> SMFLQRPKPYSDESLESFFIRVANKNGYGDVHRFLEATKRFLQDIDHNGYQTFPTDITRINPYSAKNSSSARTASFLKLAQLTFNEPPELLGLAINRTNMKYSPSTSAVVRGAEVFPRSLLRTHSIPCCPLCLRENGYASYLWHFQGYEYCHSHNVPLITTCSCGKEFDYRVSGLKGICCKCKEPITLTSRENGHEAACTVSNWLAGHESKPLPNLPKSYRWGLVHWWMGIKDSEFDHFSFVQFFSNWPRSFH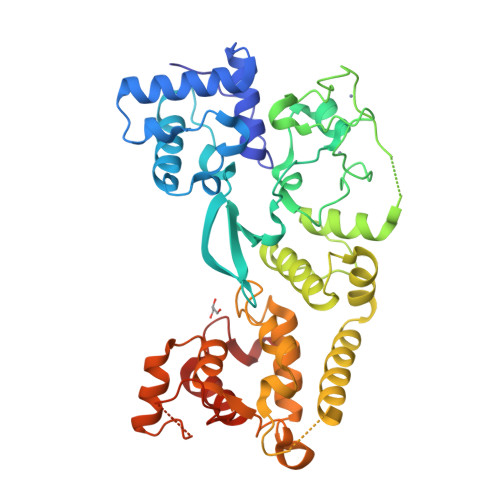SIIEDEVEFNLEHAVVSTSELRLKDLLGRLFFGSIRLPERNLQHNIILGELLCYLENRLWQDKGLIANLKMNALEATVMLNCSLDQIASMVEQRILKPNRKSKPNSPLDVTDYLFHFGDIFCLWLAEFQSDEFNRSFYVSRW> SLFAKLGGREAVEAAVDKFYNKIVADPTVSTYFSNTDMKVQRSKQFAFLAYALGGASEWKGKDMRTAHKDLVPHLSDVHFQAVARHLSDTLTELGVPPEDITD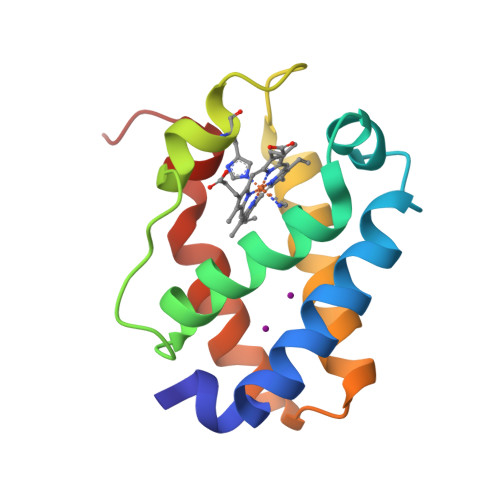AMAVVASTRTEVLNMPQQ> GSSPDKKWLGTPIEEMRRMPRCGIRLPLLRPSANHTVTIRVDLLRAGEVPKPFPTHYKDLWDNKHVKMPCSEQNLYPVEDENGERTAGSRWELIQTALLNKFTRPQNLKDAILKYNVAYSKKWDFTALIDFWDKVLEEAEAQHLYQSILPDMVKIALCLPNICTQPIPLLAAAMNHSITMSQEQIASLLANAFFCTFPRRNAKMKSEYSSYPDINFNRLFEGRSSRKPEKLKTLFCYFRRVTAAAPTGLVTFTRQSLEDFPEWERCEKPLTRLHVTYEGTIEENGQGMLQVDFANRFVGGGVTSAGLVQEEIRFLINPELIISRLFTEVLDHNECLIITGTEQYSEYTGYAETYRWSRSHEDGSERDDWQRRCTEIVAIDALHFRRYLDQFVPEKMRRELNKAYCGFLRPGVSSENLSAVATGNWGCGAFGGDARLK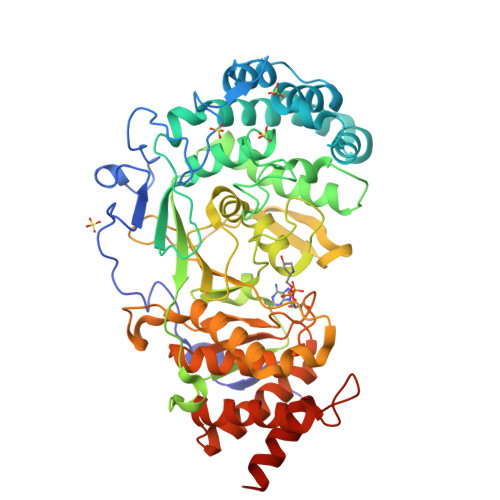ALIQILAAAAAERDVVYFTFGDSELMRDIYSMHIFLTERKLTVGDVYKLLLRYYNEECRNCSTPGPDIKLYPFIYHAVESCAETADHSGQRTGT The reduction of nitrite to form NO by nitrite reductase (NiR) is a key step in this process because it is at this point that the loss of terrestrial fixed nitrogen to the atmosphere occurs. Extensive structural studies have shown that each CuNiR monomer contains two copper sites: one type 1 copper (T1Cu) site and one type 2 copper (T2Cu) catalytic site. The T1Cu site accepts an electron from a carrier protein, either azurin or a c-type cytochrome, and in some CuNiRs these are present in an additional tethered domain. Numerous crystallographic studies of CuNiRs have shown the catalytic type 2 Cu sites to be located at the interface between adjacent monomers and to typically have a Cu–(His)3–H2O ligation.

Here, we have utilized serial femtosecond rotation crystallography (SF-ROX) using 64 large blue crystals to visualize the resting state of the active site of AxNiR, one of the most well studied CuNiRs. The sub-10 fs X-ray pulse length from the SACLA X-ray free-electron laser allowed diffraction data to be collected to 1.6 Å resolution in a ‘time-frozen’ state. The SRX structure revealed the expected water ligand bound to the catalytic T2Cu centre, while the SF-ROX structure showed an unprecedented dioxygen ligand bound to the T2Cu site in the resting state of the aerobically purified as-isolated enzyme. However, there was a large patch of positive density on top of the T2Cu in the SF-ROX model adjacent to the water molecule and the two catalytic residues. The density was clearly due to a diatomic molecule that is shifted towards the linking water position from the normal binding position of NO. The modelled O2 species perfectly fits the electron density and its bond distance was refined to 1.24 Å, which is compatible with O2/superoxide (1.2–1.3 Å) but not peroxide (1.4–1.5 Å). The O2 also has full occupancy, which is unusual for ligands bound to the T2Cu site of CuNiR. In the AxNiR SF-ROX structure, the geometry of its binding mode is unique in that it is not bound directly above the T2Cu but is translated towards the two catalytic residues. Since in our experiments the short duration (less than 10 fs) of the X-ray laser pulse precludes X-ray-induced chemistry, the SF-ROX structure obtained from the blue crystals is that of the copper(II) oxidation state. In the present case, our finding of a dioxo species bound to the T2Cu ion suggests that dioxygen reacted with a reduced NiR species at an early stage in isolation of the enzyme and represents a trapped intermediate of the oxidase reaction awaiting the delivery of a second electron to enable turnover to produce H2O2.

> DADKLPHTKVTLVAPPQVHPHEQATKSGPKVVEFTMTIEEKKMVIDDKGTTLQAMTFNGSMPGPTLVVHEGDYVQLTLVNPATNAMPHNVDFHGATGALGGAKLTNVNPGEQATLRFKADRSGTFVYHCAPEGMVPWHVVSGMSGTLMVLPRDGLKDPQGKPLHYDRAYTIGEFDLYIPKGPDGKYKDYATLAESYGDTVQVMRTLTPSHIVFNGKVGALTGANALTAKVGETVLLIHSQANRDTRPHLIGGHGDWVWETGKFANPPQRDLETWFIRGGSAGAALYTFKQPGVYAYLNHNLIEAFELGAAGHIKVEGKWNDDLMKQIKAPAPIPR> SNASQGRACLSKAELTADLIWLS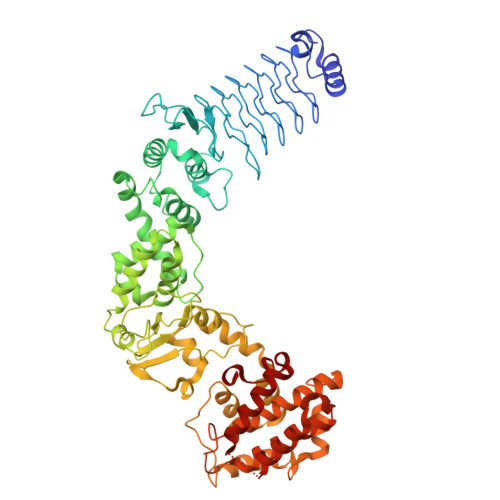ANRTGEESAEELNYSGCDLSGLSLVGLNLSSVNFSGAVLDDTDLRMSDLSQAVLENCSFKNSILNECNFCYANLSNCIIRALFENSNFSNSNLKNASFKGSSYIQYPPILNEADLTGAIIIPGMVLSGAILGDVKELFSEKSNTINLGGCYIDLSDIQENILSVLDNYTKSNKSILLTMNTSDDKYNHDKVRAAEELIKKISLDELAAFRPYVKMSLADSFSIHPYLNNANIQQWLEPICDDFFDTIMSWFNNSIMMYMENGSLLQAGMYFERHPGAMVSYNSSFIQIVMNGSRRDGMQERFRELYEVYLKNEKVYPVTQQSDFGLCDGSGKPDWDDDSDLAYNWVLLSSQDDGMAMMCSLSHMVDMLSPNTSTNWMSFFLYKDGEVQNTFGYSLSNLFSESFPIFSIPYHKAFSQNFVSGILDILISDNELKERFIEALNSNKSDYKMIADDQQRKLACVWNPFLDGWELNAQHVDMIMGSHVLKDMPLRKQAEILFCLGGVFCKYSSSDMFGTEYDSPEILRRYANGLIEQAYKTDPQVFGSVYYYNDILDRLQGRNNVFTCTAVLTDMLTEHAKESFPEIFSLYYPVAWR> MANKTYKIGKNAGYDGCGL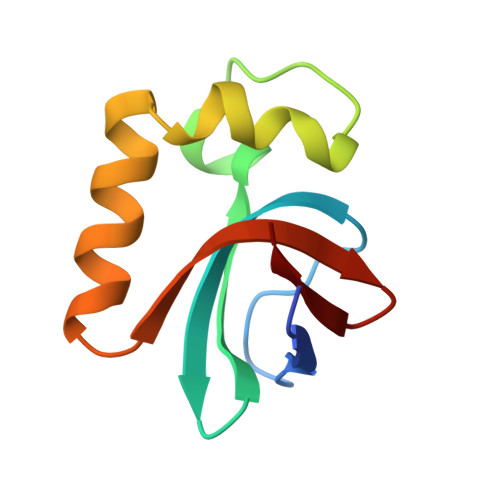CLAAISENEAIKVKYLRDICPDYDGDDKAEDWLRWGTDSRVKAAALEMEQYAYTSVGMASCWEFVEL BENZO[B]THIOPHENE-2-CARBOXAMIDINE | C9 H9 N2 S | 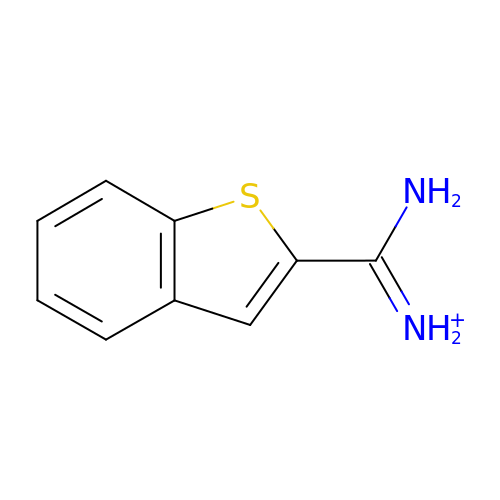JZWDLUGQTRKBNA-UHFFFAOYSA-O Bacterial cell division is a fundamental process that results in the physical separation of a mother cell into two daughter cells and involves a set of proteins known as the divisome. Early and late components are linked by the FtsQBL complex, which is well-conserved among bacteria. The FtsQBL complex may have a structural role as a scaffold in the assembly of the divisome since FtsB and FtsL proteins are recruited to the divisome by FtsQ and the resulting FtsQBL complex then recruits late divisome components. In this study, we have determined the crystal structure of the periplasmic domain of FtsQ in complex with C-terminal fragment of FtsB, showing that the C-terminal region of FtsB is a key binding region of FtsQ.

To gain further insights into structural organization of the FtsQB complex, we determined the 2.9-Å resolution structure of FtsQ50–276 bound to FtsB25–103. The electron density map of residues 25–60 was not observed for FtsB25–103, while nearly all sequences of FtsQ50–276 were found to be ordered with the exception of N- and C-terminal flexible regions (residues 50–52 and 262–276, respectively). The overall structure of FtsQ50–276 consists of two domains, α and β, and the β-domain is responsible for FtsB25–103 binding. The solvent-accessible surface area buried at the interface between FtsQ and FtsB was 1330 Å2, approximately 20% of the monomer surface area of FtsQ. The FtsB sequence (residues 61–95) folds into one α-helix (α3) and one β-strand (β1). The α-helix-turn-β-strand motif begins with the α-helix (residues 64–75), followed by a kinked loop (residues 76–82), a short β-strand (residues 83–85), and another terminal kinked loop (residues 86–95); the two kinked loops contain two proline residues (Pro80 and Pro89). The kinked loop between the α-helix (residues 64–75) and β-strand (residues 83–85) wraps around the Tyr248 residue of FtsQ. To stabilize the kinked loop conformation, four FtsB residues (Glu68, Arg72, Arg79, and Glu82) form a cluster with extensive salt-bridge networks. Interestingly, the β-strand of FtsB makes a continuous β-sheet with that of FtsQ by anti-parallel stacking with β12. The charge reversal mutations E69R, R72E, and E82R of FtsB nearly abolished binding to FtsQ. This highlights the role of FtsQ Tyr248 and the FtsB α-helix-turn-β-strand motif as affinity determinants.

> QRLPLSKLVLTGERHYTRNDDIRQSILALGEPGTFMTQDVNIIQTQIEQRLPWIKQVSVRKQWPDELKIHLVEYVPIARWNDQHMVDAEGNTFSVPPERTSKQVLPMLYGPEGSANEVLQGYREMGQMLAKDRFTLKEAAMTARRSWQLTLNNDIKLNLGRGDTMKRLARFVELYPVLQQQAQTDGKRISYVDLRYDSGAAVGWAPLPP;> NGGQEALEERARNELSMTRPGETFYRLVPDASKRA> APITAYSQQTRGLLGCIITSLTGRD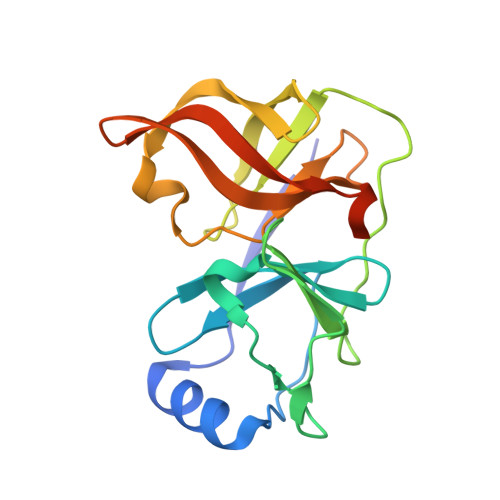KNQVDGEVQVLSTATQSFLATCVNGVCWTVYHGAGSKTLAGPKGPITQMYTNVDQDLVGWPAPPGARSMTPCTCGSSDLYLVTRHADVIPVRRRGDSRGSLLSPRPVSYLKGSSGGPLLCPSGHVVGIFRAAVCTRGVAKAVDFIPVESMETTMRSPVFTDN>[22x]MSSLLNSLLPEYFKPKTNLNINSSRVQYGFNARIDMQYEDDSGTRKGSRPNAFMSNTVAFIGNYEGIIVDDIPILDGLRADIFDTHGDLDMGLVEDALSKSTMIRRNVPTYTAYASELLYKRNLTSLFYNMLRLYYIKKWGSIKYEKDAIFYDNGHACLLNRQLFPKSRDASLESSLSLPEAEIAMLDPGLEFPEEDVPAILWHGRVSSRATCILGQACSEFAPLAPFSIAHYSPQLTRKLFVNAPAGIEPSSGRYTHEDVKDAITILVSANQAYTDFEAAYLMLAQTLVSPVPRTAEASAWFINAGMVNMPTLSCANGYYPALTNVNPYHRLDTWKDTLNHWVAYPDMLFYHSVAMIESCYVELGNVARVSDSDAINKYTFTELSVQGRPVMNRGIIVDLTLVAMRTGREISLPYPVSCGLTRTDALLQGTEIHVPVVVKDIDMPQYYNAIDKDVIEGQETVIKVKQLPPAMYPIYTYGINTTEFYSDHFEDQVQVEMAPIDNGKAVFNDARKFSKFMSIMRMMGNDVTATDLVTGRKVSNWADNSSGRFLYTDVKYEGQTAFLVDMDTVKARDHCWVSIVDPNGTMNLSYKMTNFRAAMFSRNKPLYMTGGSVRTIATGNYRDAAERLRAMDETLRLKPFKITEKLDFRVAAYAIPSLSGSNMPSLHHQEQLQISEVDAEPINPIGEDELPPDIE

L-BC virus persists in the budding yeast Saccharomyces cerevisiae, whereas other viruses from the family Totiviridae infect a diverse group of organisms including protists, fungi, arthropods, and vertebrates. Totiviridae is a family of viruses with monopartite double-stranded RNA (dsRNA) genomes, which contain two open reading frames encoding the capsid protein and the RNA-dependent RNA-polymerase (RdRp). The capsid of L-BC is organized with icosahedral symmetry with two subunits of capsid protein, named A and B, forming the icosahedral asymmetric unit. Decamers of capsid proteins are stabilized by domain swapping of the C-termini of subunits located around icosahedral fivefold axes.

Furthermore, we identified an open particle of L-BC that lacks one decamer of capsid proteins. Three-dimensional reconstruction of the open particles, with imposed fivefold symmetry, produced a 10 Å resolution capsid structure with one missing decamer of capsid proteins. The opening in the particle has a diameter of 16 nm. Overall, the structure of the open particle corresponds to that of virions and empty capsids; however, fifteen capsid proteins, two B and one A subunit from each of the five decamers that border the opening, have smeared densities indicating their high mobility. The three subunits are located further away from the particle center, and the B subunits are also shifted away from the hole. The total displacement of the border subunits is between 9 and 11 Å relative to their positions in the complete capsid. The icosahedral asymmetric unit forming the border of the opening contains fewer resolved residues than those from the remainder of the capsid. The structures of capsid proteins from the empty particle were fitted into the other reconstructions. The domain swaps of βU strands between A subunits related by a fivefold axis and the existence of open particles indicate that capsids of L-BC virus are assembled from decamers. Furthermore, the open particles may be assembly intermediates that are prepared for the incorporation of the virus (+) strand RNA.> VTAFLGERVTLTSYWRRVSLGPEIEVSWFKLGPGEEQVLIGRMHHDVIFIEWPFRGFFDIHRSANTFFLVVTAANISHDGNYLCRMKLGETEV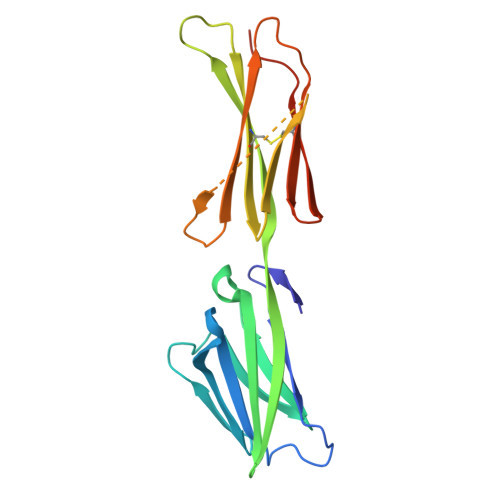TKQEHLSVVKPLTLSVHSERSQFPDFSVLTVTCTVNAFPHPHVQWLMPEGVEPAPSAANGGVMKEKDGSLSVAVDLSLPKPWHLPVTCVGKNDKEEAHGVYVSGYLSQKHHHHHH>MSTQYETQGYTINNAGRRLVVDPITRIEGHMRCEVNINDQNVITNAVSCGTMFRGLEIILQGRDPRDAWAFVERICGVCTGVHALASVYAIEDAIGIKVPDNANIIRNIMLATLWCHDHLVHFYQLAGMDWIDVLDALKADPRKTSELAQSLSSWPKSSPGYFFDVQNRLKKFVEGGQLGIFRNGYWGHPQYKLPPEANLMGFAHYLEALDFQREIVKIHAVFGGKNPHPNWIVGGMPCAINIDESGAVGAVNMERLNLVQSIITRTADFINNVMIPDALAIGQFNKPWSEIGTGLSDKCVLSYGAFPDIANDFGEKSLLMPGGAVINGDFNNVLPVDLVDPQQVQEFVDHAWYRYPNDQVGRHPFDGITDPWYNPGDVKGSDTNIQQLNEQERYSWIKAPRWRGNAMEVGPLARTLIAYHKGDAATVESVDRMMSALNLPLSGIQSTLGRILCRAHEAQWAAGKLQYFFDKLMTNLKNGNLATASTEKWEPATWPTECRGVGFTEAPRGALGHWAAIRDGKIDLYQCVVPTTWNASPRDPKGQIGAYEAALMNTKMAIPEQPLEILRTLHSFDPCLACSTH[2x];>LENKPRIPVVWIHGLECTCCTESFIRSAHPLAKDVILSLISLDYDDTLMAAAGTQAEEVFEDIITQYNGKYILAVEGNPPLGEQGMFCISSGRPFIEKLKRAAAGASAIIAWGTCASWGCVQAARPN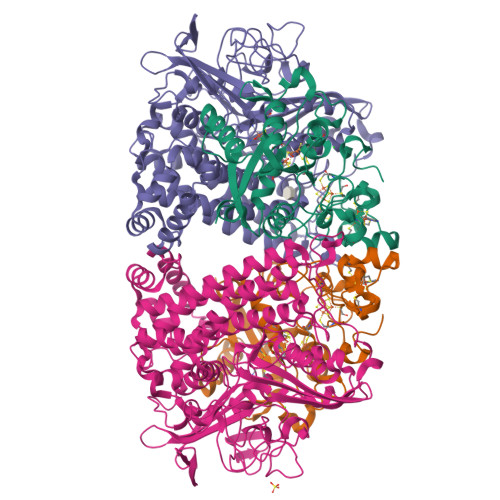PTQATPIDKVITDKPIIKVPGCPPIPDVMSAIITYMVTFDRLPDVDRMGRPLMFYGQRIHDKCYRRAHFDAGEFVQSWDDDAARKGYCLYKMGCKGPTTYNACSSTRWNDGVSFPIQSGHGCLGCAENGFWDRGSFYSRVVDIPQMGTHSTADTVGLTALGVVAAAVGVHAVASAVDQRRRHNQQPTETEHQPGNEDKQARSHHHHHH[2x]> MGRIISIVSGKGGTGKTTVTANLSVALGD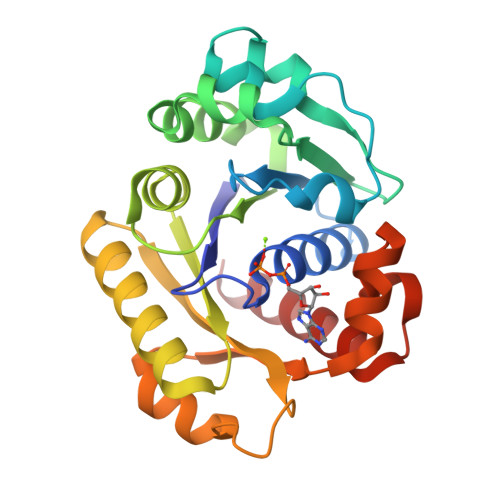RGRKVLAVDGDLTMANLSLVLGVDDPDVTLHDVLAGEANVEDAIYMTQFDNVYVLPGAVDWEHVLKADPRKLPEVIKSLKDKFDFILIDCPAGLQLDAMSAMLSGEEALLVTNPEISCLTDTMKVGIVLKKAGLAILGFVLNRYGRSDRDIPPEAAEDVMEVPLLAVIPEDPAIREGTLEGIPAVKYKPESKGAKAFVKLAEEIEKLA>[4x]MAQLTTESMPFNVAEGKEVLLL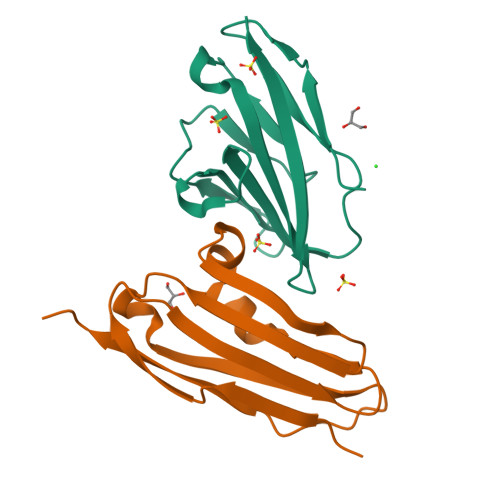VHNLPQQLFGYSWYKGERVDGNRQIVGYAIGTQQATPGPANSGRETIYPNASLLIQNVTQNDTGFYTLQVIKSDLVNEEATGQFHVY;>TAPTLTVTPEQQTVKVDEDITFTVTVEDENEVELGLDDLKAKYENDIIGARVKIKYLTKEPNKKVMEVTIMKATLADKGAITFTAKDKAGNQAEPKTVTINVLPLKDSNEPKLPSTGGSHHHHHH[4x]Of these, kust_36903, hereafter designated Ks-Amt5, uniquely features an extended, cytoplasmic domain with high homologies to histidine kinases (HK) of the HisKA subfamily. Ks-Amt5 is a 679 amino-acid protein organized into an N-terminal ammonium transport (Amt) domain connected to a C-terminal domain of 269 residues. Ks-Amt5 represents the prototype of a modular sensor-transducer system that evolved from the widespread ammonium transporter role to serve as a specific receptor for the NH4+ cation. We find that the canonical ammonium transporter module in Ks-Amt5, has been repurposed to selectively bind ammonium cations in a binding pocket that is not present in orthologues described previously.

Ks-Amt5 crystallized in space group P63 and crystals diffracted to a resolution better than 2 Å using synchrotron radiation. The structure was solved and refined to 1.98 Å resolution, but only the transmembrane Amt domain was well defined in the electron density maps. The detailed atomic model covered amino-acid residues 1–405 up to the beginning of the helical connector between the two domains. From here on, the quality of the electron density map deteriorated due to structural disorder of the HK domain, and although various features such as extended helices were discernible, an atomic model could not be built. The transmembrane domain of Ks-Amt5 follows the Amt/Rh fold, aligning to A. fulgidus Amt1 with a root-mean-squared deviation of all-atom positions of 1.2 Å. As expected from primary structure alignments, all known functional motifs are retained, including the selectivity filter (W144, S227), the Phe gate (F103, F223) and the His pair (H171, H326). Here, two ammonium cations are tightly coordinated by a network of residues, namely Q24 and E31 from helix h1, N47, D50 and T51 from h2 and T109 and T112 from h4. The observed binding geometry with five ligands on each cation is distinct from the octahedral symmetry commonly observed for Na+, and the short bond distances of 2.2–2.4 Å are in excellent agreement with calculated and observed coordination distances of water to NH4+, making the assignment unambiguous. Ks-Amt5 thus diverts the substrate cations that have passed the selectivity filter (W144, S227) into high-affinity binding sites, where binding may lead to structural rearrangements that trigger signaling.

> MENIQININHLWVIMAACMVFLMQLGFTSYETGFSQSKNAISIALRNLVDTLISSLVFFSVGFGFMFGKSYMGLIGIDLFFANDLALHPNTLSYSFFFFQMVFASTAATILTGAIAERSGFIPNIAGTAFIVAIIYPIFGHWAWGNLFSPDQTGWLKELGFIDFAGATVVHSIGGWFAMAAAIMVGPRIDKYNPDGSSNRIGLHNVPLATLGTFFLWFGWFGFNGGSLLRVSVNIGLVILNTNMAAASAGVSALIFIYATRKRIEAGSLFTAILAGLVAITASSNMVTPVSAVAIGLITGILAIIAEGFIEKTLKIDDPVSAIAVHGVGGVIGTLCVAIFAQKSYLLAENGSRMHQLGIQALGVIVAFSWSFGLGMLFFLCLKKVKRLRVTPEEEKRGLNVAEAA>MSLEGFICKFNRKRRLYIENIMQVRVTGILIEDEKVLLVKQKVANRDWSLPGGRVENGETLEEAMIREMREETGLEVKIKKLLYVCDKPDASPSLLHITFLLERIEGEITLPSNEFDHNPIHDVQMVPINELSYYGFSETF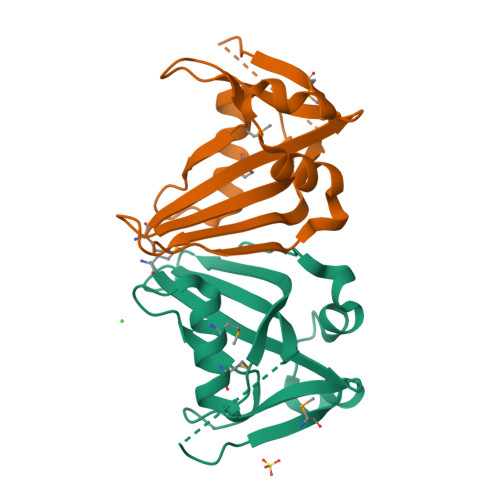INLISGGLANAGSYQGLKRNIGEGHHHHHH[2x]> MNSPISPIETVPVKLKPGMDGPKVKQWPLTEEKIKALVEICTEMEKEGKISKIGPENPYNTPVFAIKKKDSTKWRKLVDFRELNKRTQDFWEVQLGIPHPAGLKKKKSVTVLDVGDAYFSVPLDEDFRKYTAFTIPSINNETPGIRYQYNVLPQGWKGSPAIFQSSMTKILEPFRKQNPDIVIC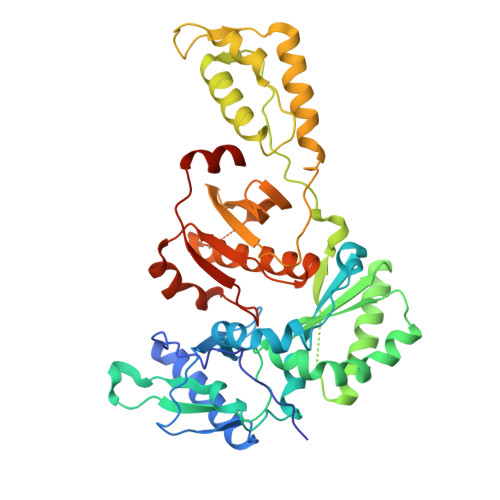QYMDDLYVGSDLEIGQHRTKIEELRQHLLRWGLTTPDKKHQKEPPFLWMGYELHPDKWTVQPIVLPEKDSWTVNDIQKLVGKLNWASQIYPGIKVRQLCKLLRGTKALTEVIPLTEEAELELAENREILKEPVHGVYYDPSKDLIAEIQKQGQGQWTYQIYQEPFKNLKTGKYARMRGAHTNDVKQLTEAVQKITTESIVIWGKTPKFKLPIQKETWETWWTEYWQATWIPEWEFVNTPPLVKLWYQLEKEPIVGAETF> DTFPGTNGLDFTIDGTAGYFAGSNAYWLAFLTNNDDVDKVLGDAESSGLRIMRVWGFNDVNTVPSSGTVYFQLLQDG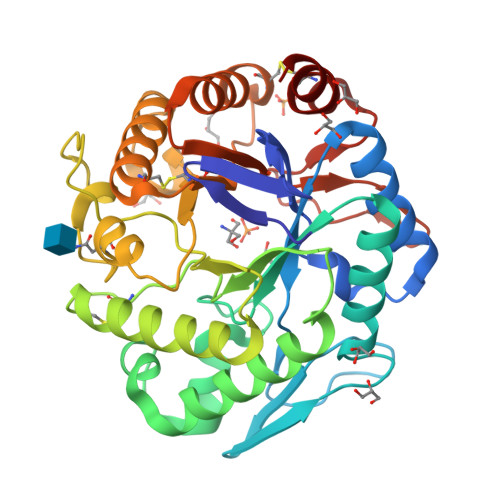TATINTGSDGLERLDYVVSSAEQHNVKLIINFVNNWSDYGGIPAYVNAFGGSTTSWYTDEASQAAYRNYIKTVVSRYIDSPAVFAWELANEPRCHGCDTSVIYNWVAATSSFIKSIDSQHLVCIGDEGLGLDIDSDGSYPYSYYEGTNFTLNLGVDTIDFGTFHLYPSSWGVSNSFGSPWVTAHGAACAAAGKPCLFEEYGVTSDKCSVEGGWQQTALDTRGIGADSFWQFGDTLSTGQSPNDGYTIYYGTDDYTCLVTDRVASI> GSILDPEVLKVAEYVYQERLSKPYTEV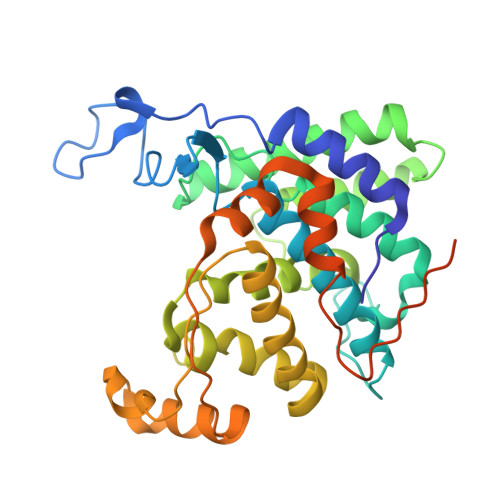GPEWEYNHKTPYATRATGTGHNLQRFITIDDQRLHRPIHGLAHTMRTLFYSQLMYEAAKRQPHPHRCADGRTIADLSVQDLKKLNIAQLFFVAGRESEASYGDAYHRYHLYGAKQFEAYARKHLTHLFSEKEIVLYSRCIEDRIGDRFDETAEGYLIHLSHMIDLMRCKSPVEVFIGHSRGVSGIVPTLIQLFGREDGLDIMHYARSLFAATGEAVPYISSSEWPHLGIESDRVERALKIVGSLEVEGQEADAKKTAQAGFSVDGCYGALVKIDTPDWYHQVKEKEDYDVDEVIALPPQITIREEPPKTNESFLLSL> PAGIIPTGNVLSTIEVCAHRCIFDFFKQIRSDDNSLYSAQFDILLGTYCNTLNFVRFLELGLSVACICTKFPELAYVRDGVIQFEVQQPMIARDGPHPVDQPVHNYMVKRIHKRSLSAAFAIASEALSLLSNTYVDGTEIDSSLRIRAIQQMARNLRTVLDSFERGTADQLLGVLLEKAPPLSLLSPINKFQPEGHLNRVARAALLSDLKRRVCADMFFMTRHAREPRLISAYLSDMVSCTQPSVMVSRITHTNTRGRQVDGVLVTTATLKRQLLQGILQIDDTAADVPVTYGEMVLQGTNLVTALVMGKAVRGMDDVARHLLDITDPNTLNIPSIPPQSNSDSTTAGLPVNARVPADLVIVGDKLVFLEALERRVYQATRVAYPLIGNIDITFIMPMGVFQANSMDRYTRHAGDFSTVSEQDPRQFPPQGIFFYNKDGILTQLTLRDAMGTICHSSLLDVEATLVALRQQHLDRQCYFGVYVAEGTEDTLDVQMGRFMETWADMMPHHPHWVNEHLTILQFIAPSNPRLRFELNPAFDFFVAPGDVDLPGPQRPPEAMPTVNATLRIINGNIPVPLCPISFRDCRGTQLGLGRHTMTPATIKAVKDTFEDRAYPTIFYMLEAVIHGNERNFCALLRLLTQCIRGYWEQSHRVAFVNNFHMLMYITTYLGNGELPEVCINIYRDLLQHVRALRQTITDFTIQGEGHNGETSEALNNILTDDTFIAPILWDCDALIYRDEAARDRLPAIRVSGRNGYQALHFVDMAGHNFQRRDNVLIHGRPVRGDTGQAIPITPHHDREWGILSKIYYYIVIPAFSRGSCCTMGVRYDRLYPALQAVIVPEIPADEEAPTTPEDPRHPLHAHQLVPNSLNVYFHNAHLTVDGDALLTLQELMGDMAERTTAILVSSAPDAGAATATTRNMRIYDGALYHGLIMMAYQAYDETIATGTFFYPVPVNPLFACPEHLASLRGMTNARRVLAKMVPPIPPFLGANHHATIRQPVAYHVTHSKSDFNTLTYSLLGGYFKFTPISLTHQLRTGFHPGIAFTVVRQDRFATEQLLYAERASESYFVGQIQVHHHDAIGGVNFTLTQPRAHVDLGVGYTAVCATAALRCPLTDMGNTAQNLFFSRGGVPMLHDNVTESLRRITASGGRLNPTEPLPIFGGLRPATSAGIARGQASVCEFVAMPVSTDLQYFRTACNPRGRASGMLYMGDRDADIEAIMFDHTQSDVAYTDRATLNPWASQKHSYGDRLYNGTYNLTGASPIYSPCFKFFTPAEVNTNCNTLDRLLMEAKAVASQSSTDTEYQFKRPPGSTEMTQDPCGLFQEAYPPLCSSDA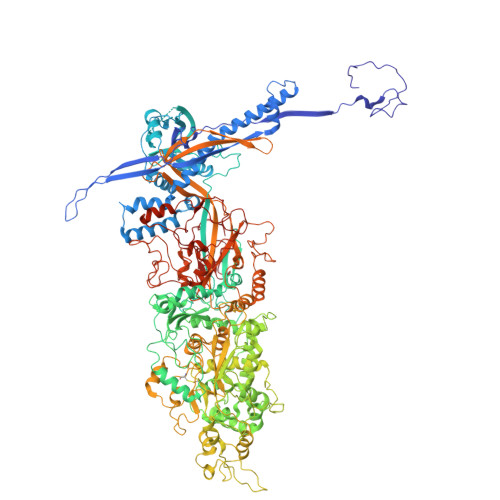AMLRTAHAGETGADEVHLAQYLIRDASPLRGCLPL Human mitochondrial gene expression relies on the specific recognition and aminoacylation of mitochondrial tRNAs (mtRNAs) by nuclear-encoded mitochondrial aminoacyl-tRNA synthetases (mt-aaRSs). Here, we present cryo-EM structures of the human mitochondrial seryl-tRNA synthetase (mSerRS) in complex with mtRNASer(GCU). The mtRNASer(GCU) is highly degenerated, having lost the entire D-arm, tertiary core, and stable L-shaped fold that define canonical tRNAs. Instead, mtRNASer(GCU) evolved unique structural innovations, including a radically altered T-arm topology that serves as critical identity determinant in an unusual shape-selective readout mechanism by mSerRS.

To understand the molecular basis for tRNA-recognition in human mitochondria, we first determined the high-resolution crystal structure of human mSerRS bound to 5’-O-[N-(L-seryl)sulfamoyl] adenosine (SerSA), a non-hydrolysable analog of the seryl-adenylate intermediate. Appended to each catalytic domain is an N-terminal domain, which forms a long coiled-coil ‘helical arm’ of two antiparallel α-helices that protrudes away from the synthetase core. Both active sites are occupied by a SerSA molecule, bound similar to previously described SerRS structures.

>[2x]TTEKRNRNLLYEYAREGYSALPQLDIERFCACPEEAAHALELRKGELRSADLPAIISTWQELRQLQEQIRSLEEEKAAVTEAVRALLANQDSGEVQQDPKYQGLRARGREIRKELVHLYPREAQLEEQFYLQALKLPNQTHPDVPVGDESQARVLHMVGDKPVFSFQPRGHLEIGEKLDIIRQKRLSHVSGHRSYYLRGAGALLQHGLVNFTFNKLLRRGFTPMTVPDLLRGAVFEGCGMTPNANPSQIYNIDPARFKDLNLAGTAEVGLAGYFMDHTVAFRDLPVRMVCSSTCYRAETNTGQEPRGLYRVHHFTKVEMFGVTGPGLEQSSQLLEEFLSLQMEILTELGLHFRVLDMPTQELGLPAYRKFDIEAWMPGRGRFGEVTSASNCTDFQSRRLHIMFQTEAGELQFAHTVNATACAVPRLLIALLESNQQKDGSVLVPPALQSYLGTDRITAPTHVPLQYIGPNQPRKPGLPGQPAVS>MQKYSKLMADSIIAKNITLTDHWGYEYGLTLDGIAKVYEWTKDKKYLDFIIKTM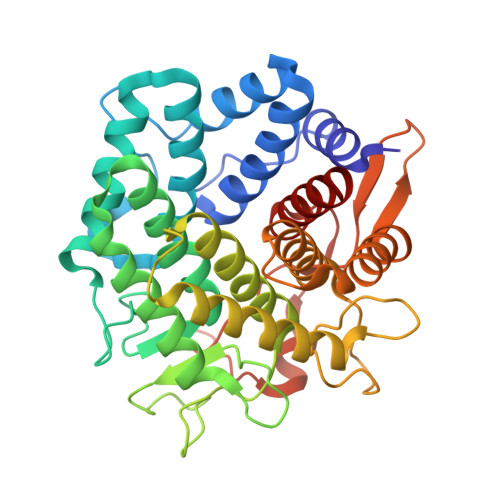DTFINEDGTINGYKLEEYNIDHLNNGKILITLFKETGKEKYRKALINLRKQIDNHPRTKENVFWHKNIYPHQIWLDGLYMGATFYAKYVKEFGEEKEFDDITHQFIITEKNLKDNKTGLLYHAYDESKTEPWSNSETGLSPHFWGRAMGWYVMALADTIEVLPKNHKDRNALIKILNNCVTALLKVQDNASKVWYQVLDEGERKGNYLEASGSSMIVYALLKGVRLGYLPESLKETAKEAYKGLINEFILETKDGLINLNKICYVAGLGGKDKRDGSFAYYISEPIVSNEPKGLGPFLLASYEYETL[2x]>[2x]MSKTQEFRPL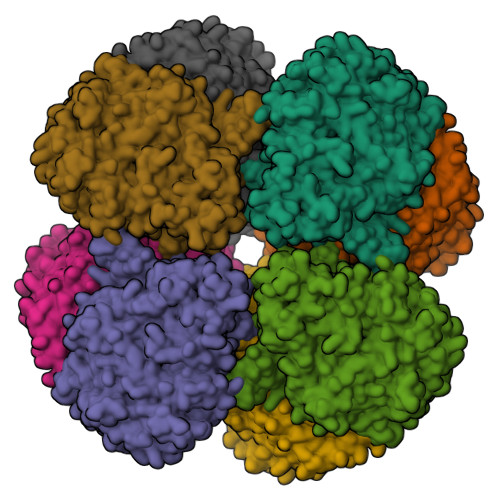TLPPKLSLSDFNEFIQDIIRIVGSENVEVISSKDQIVDGSYMKPTHTHDPHHVMDQDYFLASAIVAPRNVADVQSIVGLANKFSFPLWPISIGRNSGFGGAAPRVSGSVVLDMGKNMNRVLEVNVEGAYCVVEPGVTYHDLHNYLEANNLRDKLWLDVPDLGGGSVLGNAVERGVGYTPYGDHWMMHSGMEVVLANGELLRTGMGALPDPKRPETMGLKPEDQPWSKIAHLFPYGFGPYIDGLFSQSNMGIVTKIGIWLMPNPRGYQSYLITLPKDGDLKQAVDIIRPLRLGMALQNVPTIRHILLDAAVLGDKRSYSSRTEPLSDEELDKIAKQLNLGRWNFYGALYGPEPIRRVLWETIKDAFSAIPGVKFYFPEDTPENSVLRVRDKTMQGIPTYDELKWIDWLPNGAHLFFSPIAKVSGEDAMMQYAVTKKRCQEAGLDFIGTFTVGMREMHHIVCIVFNKKDLIQKRKVQWLMRTLIDDCAANGWGEYRTHLAFMDQIMETYNWNNSSFLRFNEVLKNAVDPNGIIAPGKSGVWPSQYSHVTWKL> GHMNVKRRTHNVLE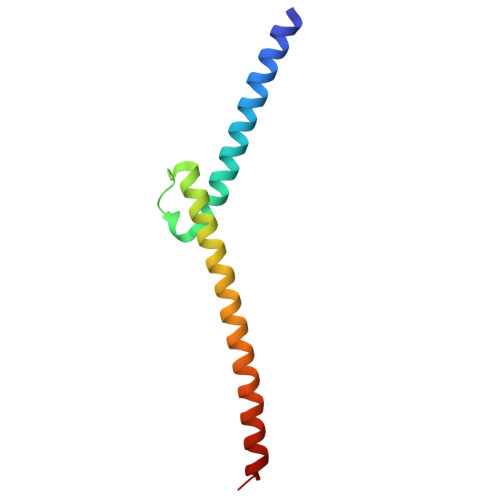RQRRNELKRSFFALRDQIPELENNEKAPKVVILKKATAYILSVQAEEQKLISEEDLLRKRREQLKHKLEQLGGC>MSAIALYLEINKLRLKIDEPMQLAIWPQLFPLLCDEHQSVQLNTDVLINFMMHVARKSQNTILNNNAAIASQYAAGNADVVAAPASAQPTPRPVINLFARANAAAPAQPSEELINMRRYRNAARKLIHHYSLNSTSSTEYKISDVVMTMIFLLRSEKYHSLFKLLETTFDDYTCRPQMTQVQTDTLLDAVRSLLEMPSTTIDLTTVDIMRSSFARCFNSPIMRYAKIVLLQNVALQRDKRTTLEELLIERGEKIQMLQPQQYINSGTEIPFCDDAEFLNRLLKHIDPYPLSRMYYNAANTMFYTTMENYAVSNCKFNIEDYNNIFKVMENIRKHSNKNSNDQDELNIYLGVQSSNAKRKKY[2x];>MKRIKCNKVRTVTEIVNSDEKIQKTYELAEFDLKNLSSLESYETLKIKLALSKYMAMLSTLEMTQPLLEIFRNKADTRQIAAVVFSTLAFIHNRFHPLVTNFTNKMEFVVTETNDTSIPGEPILFTENEGVLLCSVDRPSIVKMLSREFDTEALVNFENDNCNVRIAKTFGASKRKNTTRS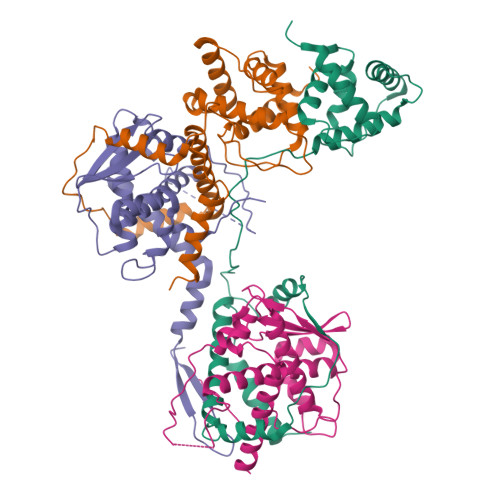DDYESNKQPNYDMDLSDFSITEVEATQYLTLLLTVEHAYLHYYIFKNYGVFEYCKSLTDHSLFTNKLRSTMSTKTSNLLLSKFKFTIEDFDKINSNSVTSGFNIYNFNK[2x]> ALWQFNGMIKCKIPSSEPLLDFNNYGCYCGLGGSGTPVDDLDRCCQTHDNCFKQ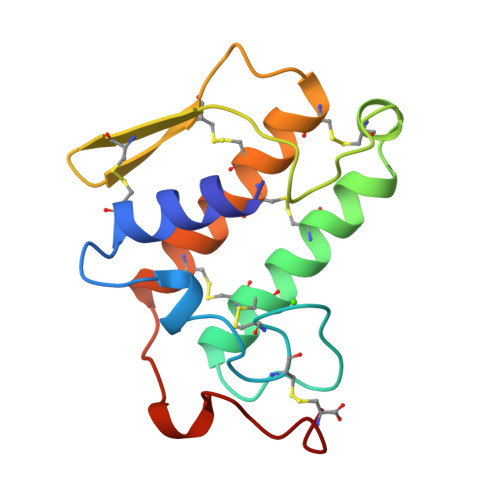AKKLDSCKVLVDNPYTNNFSYSCSNNEITCSSENNACEAFICNCNRNAAICFSKVPYNKEHKNLDKKNC4-(dimethylamino)-N-{[4-(hydroxycarbamoyl)phenyl]methyl}-N-{2-[(4-methylphenyl)amino]-2-oxoethyl}benzamide 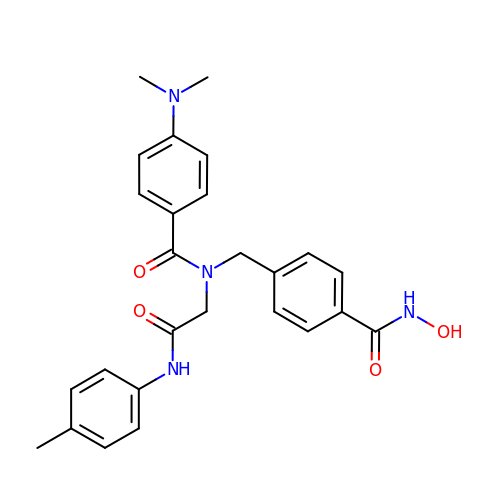| C26 H28 N4 O4 | UEKPDDMOEDHDCS-UHFFFAOYSA-N> SMLGERRRGLTDPEMAEVILKALPEAPLDGNNKMGYFVTPRWKRLTEYEALTVYAQPNADWIAGGLDWGDWTQKFHGGRPSWGNETTELRTVDWFKHRDPLRRWHAPYVKDKAEEWRYTDRFLQGYSADGQIRAMNPTWRDEFINRYWGAFLFNEYGLFNAHSQGAREALSDVTRVSLAFWGFDKIDIAQMIQLERGFLAKIVPGFDESTAVPKAEWTNGEVYKSARLAVEGLWQEVFDWNESAFSVHAVYDALFGQFVRREFFQRLAPRFGDNLTPFFINQAQTYFQIAKQGVQDLYYNCLGDDPEFSD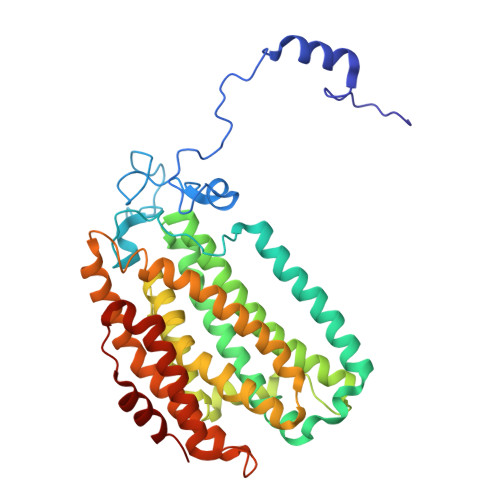YNRTVMRNWTGKWLEPTIAALRDFMGLFAKLPAGTTDKEEITASLYRVVDDWIEDYASRIDFKADRDQIVKAVLAGLK>[3x]EERRRRAAAVIEEVEQRFSTPTALLRGIADAMVEEMERGLRADPHAPLKMLISYVDNLPTGDEHGLFYALDLGGTNFRVIRVQLGGREKRVVSQQYEEVAIPPHLMVGTSMELFDFIAAELESFVKTEGEDFHLPEGRQRELGFTFSFPVHQTSISSGTLIKWTKGFSINGTVGEDVVAELSRAMERQGLDMKVTALVNDTVGTLAGGRYVDNDVAAAVILGTGTNAAYVEHANA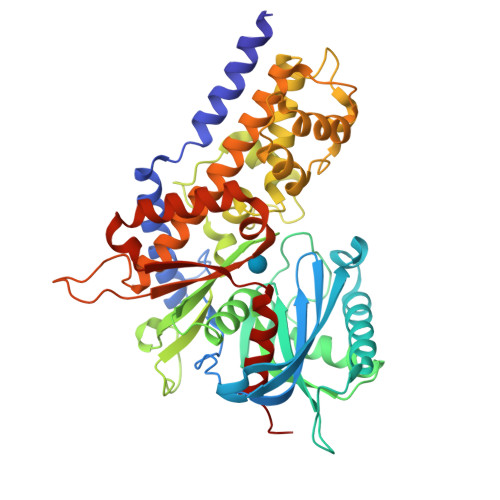IPKWTGLLPRSGNMVINMEWGNFKSERLPRSDYDNALDFESLNPGEQIYEKMISGMYLGEIVRRILLKLAHDASLFGDVVPTKLEQRFILRTPDMSAMHHDTSHDLKHLGAKLKDILGVADTSLEARYITLHVCDLVAERGARLAAAGIYGILKKLGRDRVPSDGSQKQRTVIALDGGLYEHYKKFRTCLEATLADLLGEEAASSVVVKLANDGSGIGAALLAASHSQYA> MHHHHHHHHHHSGDEV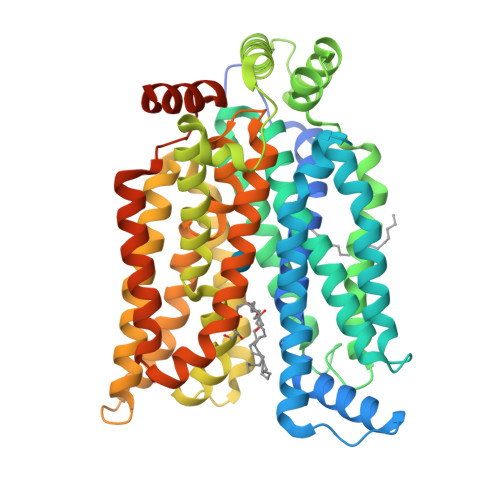DAGSGQVDAGTMGTQKVTPALIFAITVATIGSFQFGYNTGVINAPEKIIKEFITKTLTDKGNAPPSEVLLTSLWWLSVAIFSVGGMIGSFSVGLFVNRFGRRNSMLIVNLLAVTGGCFMGLCKVAKSVEMLILGRLVIGLFCGLCTGFVPMYIGEISPTALRGAFGTLNQLGIVVGILVAQIFGLEFILGSEELWPLLLGFTILPAILQSAALPFCPESPRFLLINRKEEENAKQILQRLWGTQDVSQDIQEMKDESARMSQEKQVTVLELFRVSSYRQPIIISIVLQLSQQLSGINAVFYYSTGIFKDAGVQEPWYATIGAGVVNTIFTVVSLFLVERAGRRTLHMIGLGGMAFCSTLMTVSLLLKDNYNGMSFVCIGAILVFVAFFEIGPGPIPWFIVAELFSQGPRPAAMAVAGCSNWTSNFLVGLLFPSAAHYLGAYVFIIFTGFLITFLAFTFFKVPETRGRTFEDITRAFEGQAHGADRSGKDGVMEMNSIEPAKETTTNV> HHHHHHGGGGSGGGGSGVKGAKGYRGPEGPQGPPGHQGPPGPDECEILDIIMKMCSCCECKCGPIDLLFVLDSSESIGLQNFEIAKDFVVKVIDRLSRDELVKFEPGQSYAGVVQYSHSQMQEHVSLRSPSIRNVQELKEAIKSLQWMAGGTFTGEALQYTRDQLLPPSPNNRIALVITDGRSDTQRDTTPLNVLCSPGIQVVSVGIKDVFDFIPGSDQLNVISCQGLAPSQGRPGLSLVKENYAELLEDAFLKNVTAQICIDKKCPDYTCPITFSSPADITILLDGSASVGSHNFDTTKRFAKRLAERFLTAGRTDPAHDVRVAVVQYSGTGQQRPERASLQFLQNYTALASAVDAMDFINDATDVNDALGYVTRFYREASSGAAKKRLLLFSDGNSQGATPAAIEKAVQEAQRAGIEIFVVVVGRQVNEPHIRVLVTGKTAEYDVAYGESHLFRVPSYQALLRGVFHQTVSRKVALG;> SAWSHPQFEKGGGGSGGGGSGEPGPRGPRGVPGPEGEPGPPGDPGLTECDVMTYVRETCGCCDCEKRCGALDVVFVIDSSESIGYTNFTLEKNFVINVVNRLGAIAKDPKSETGTRVGVVQYSHEGTFEAIQLDDEHIDSLSSFKEAVKNLEWIAGGTWTPSALKFAYDRLIKESRRQKTRVFAVVITDGRHDPRDDDLNLRALCDRDVTVTAIGIGDMFHEKHESENLYSIACDKPQQVRNMTLFSDLVAEKFIDDMEDVLCPDPQIVCPDLPCQTELSVAQCTQRPVDIVFLLDGSERLGEQNFHKARRFVEQVARRLTLARRDDDPLNARVALLQFGGPGEQQVAFPLSHNLTAIHEALETTQYLNSFSHVGAGVVHAINAIVRSPRGGARRHAELSFVFLTDGVTGNDSLHESAHSMRNENVVPTVLALGSDVDMDVLTTLSLGDRAAVFHEKDYDSLAQPGFFDRFIRWIC;> DYKDDDDKGGGGSGGGGSGPPGIVGQKGRPGYPGPAGPRGNRGDSIDQCALIQSIKDKCPCCYGPLECPVFPTELAFALDTSEGVNQDTFGRMRDVVLSIVNVLTIAESNCPTGARVAVVTYNNEVTTEIRFADSKRKSVLLDKIKNLQVALTSKQQSLETAMSFVARNTFKRVRNGFLMRKVAVFFSNTPTRASPQLREAVLKLSDAGITPLFLTRQEDRQLINALQINNTAVGHALVLPAGRDLTDFLENVLTCHVCLDICNIDPSCGFGSWRPSFRDAAAAGSDVDIDMAFILDSAETTTLFQFNEMKKYIAYLVRQLDMSPDPKASQHFARVAVVQHAPSESVDNASMPPVKVEFSLTDYGSKEKLVDFLSRGMTQLQGTRALGSAIEYTIENVFESAPNPRDLKIVVLMLTGEVPEQQLEEAQRVILQAKCKGYFFVVLGIGRKVNIKEVYTFASEPNDVFFKLVDKSTELNEEPLMRFGRLLPSFV

Collagen VI links the cell surface to the extracellular matrix to provide mechanical strength to most mammalian tissues, and is linked to human diseases including muscular dystrophy, fibrosis, cardiovascular disease and osteoarthritis. Collagen VI assembles from heterotrimers of three different α-chains into microfibrils, but there are many gaps in our knowledge of the molecular assembly process. All collagen VI chains have a short collagenous region flanked by globular N and C-termini, which are mainly composed of domains homologous to the A-domains of Von Willebrand factor (vWA)2. Collagen VI assembles in a hierarchical manner where three collagen VI α-chains associate to form heterotrimers.

Therefore, to understand how collagen VI monomers assemble, an expression system was designed to generate mini-collagen VI heterotrimers with the C-terminal domains of the α1, α2 and α3 chains and a short stretch of collagenous sequence with nine Gly-X-Y triplets. Processing of the cryoEM data revealed that there was substantial flexibility between the vWA domains, presumably due to the interdomain linkers, but a core of three vWA domains could be resolved, with additional diffuse areas of density, likely to be the other three vWA domains, seen in the 2D classes. Local refinements of the most structurally homogenous region yielded a 3.14 Å resolution structure, with additional diffuse areas of density for the other three vWA domains seen at higher thresholds. The three vWA domains, which were resolved to high resolution, were the α3 C1 and C2 domains and the α2 C2 domain, where the α3 C2 domain is adjacent to the α3 C1 domain. The trimeric coiled coil has hydrophobic amino acids involved in stabilising the internal surface. The coiled coil is stabilised by two interchain disulphide bonds between α3 and α2, and α2 and α1 chains. The α3 C1 domain packs closely against the coiled coil, with Tyr597 from the α2 chain coiled coil contributing to a hydrophobic pocket with residues Ile2380, Phe2399 and Phe2506, which likely stabilises the interface. The opposite side of the α3 C1 domain interacts with the α2 C2 domain, where salt bridges are formed between residues Asp2462 and Arg965 and Arg 2501 and Glu941. The mini-collagen VI structure shows how this occurs for collagen VI, as there is a short region of the collagenous triple-helical domain visible in the structure emerging from the coiled coil region. The interchain hydrogen bonds and stagger suggest that the α3 chain is trailing, the α2 chain is the middle and the α1 chain is leading, going from a C- to N-terminal direction using the convention defined in ref.>[2x]MEIISPIITPFDKQGKVNVDALKTHAKNLLEKGIDAIFVNGTTGLGPALSKDEKRQNLNALYDVTHKLIFQVGSLNLNDVMELVKFSNEMDILGVSSHSPYYFPRLPEKFLAKYYEEIARISSHSLYIYNYPAATGYDIPPSILKSLPVKGIKDTNQD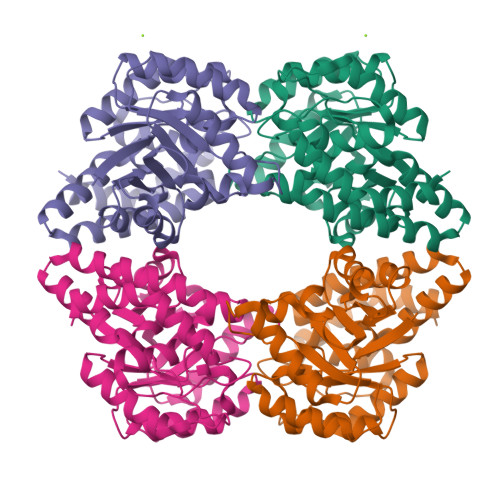LAHSLEYKLNLPGVKVYNGSNTLIYYSLLSLDGVVASFTNFIPEVIVKQRDLIKQGKLDDALRLQELINRLADILRKYGSISAIYVLVNEFQGYDVGYPRPPIFPLTDEEALSLKREIEPLKRKIQELVH>MTYSAENTEVYITSQQLEQAVTRLAEQINQDYSGQQVTLVCVLKGSFMFFADLVRKLRIDLRTQFITASSYGSSTKSSGTVTLTET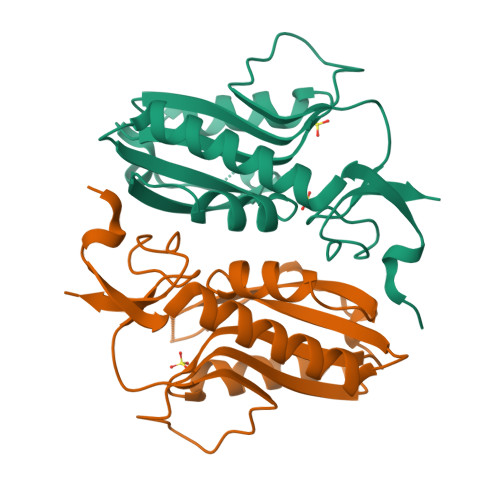SLKEEYVKDKNIIIIEDIVDTGHTYHKLIEGIGKYNPKTLKFATLLFKPARLERDVKLDYVCFEIEDKFIVGYGLDFDEKYRELPYIGLIK[4x]> SNAMNKVHFVGAGPGDKELITLKGYKLLSNADVVIYAGSLVNPELLEYCKEDCQIHNSAHMDLQEIIDVMREGIENNKSVVRLQTGDFSIYGSIREQVEDLNKLNIDYDCTPGVSSFLGAASSLGVEYTVPEISQSVIITRMEGRTPVPEKESIQSYAKHQTSMVIFLSVQEIEKVVSKLLEGGYPKDTPIA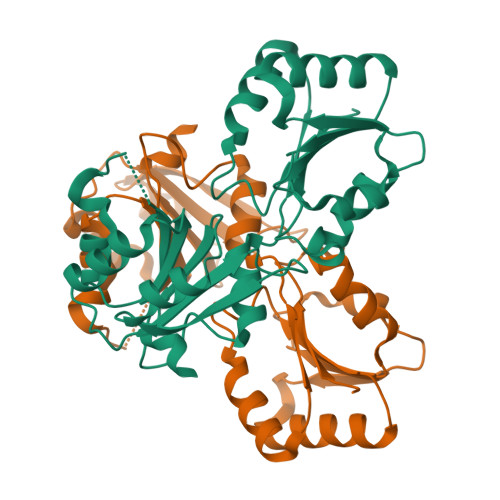VIYKATWADEKIVKGTLSDIAVKVKENNINKTALIMVGRFLGEEYNNSKLYDKDFKHEYRG>MLVFIDDGSTNIKLQWQESDGTIKQHISPNSFKREWAVSFGDKKVFNYTLNGEQYSFDPISPDAVVTTNIAWQYSDVNVVAVHHALLTSGLPVSEVDIVCTLPLTEYYDRNNQPNTENIERKKANFRKKITLNGGDTFTIKDVKVMPESIPAGYEVLQELDELDSLLIIDLGGTTLDISQVMGKLSGISKIYGDSSLGVSLVTSAVKDALSLARTKGSSYLADDIIIHRKDNNYLKQRINDENKISIVTEAMNEALRKLEQ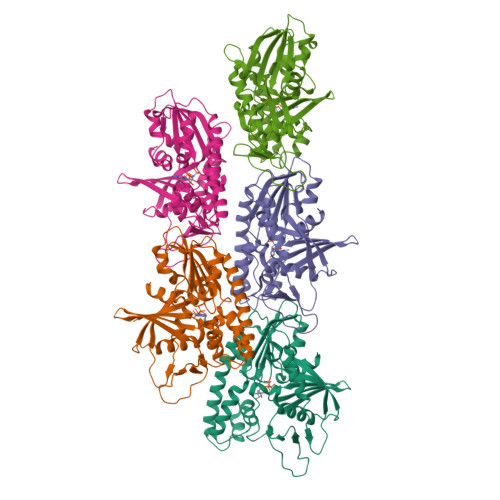RVLNTLNEFSGYTHVMVIGGGAELICDAVKKHTQIRDERFFKTNNSQYDLVNGMYLI[5x]> MAAPEAEVLSSAAVPDLEWYEKSEETHASQIELLETSSTQEPLNASEAFCPRDCMVPVVFPGPVSQEGCCQFTCELLKHIMYQRQQLPLPYEQLKHFYRKPSPQAEEMLKKKPRATTEVSSRKCQQALAELESVLSHLEDFFARTLVPRVLILLGGNALSPKEFYELD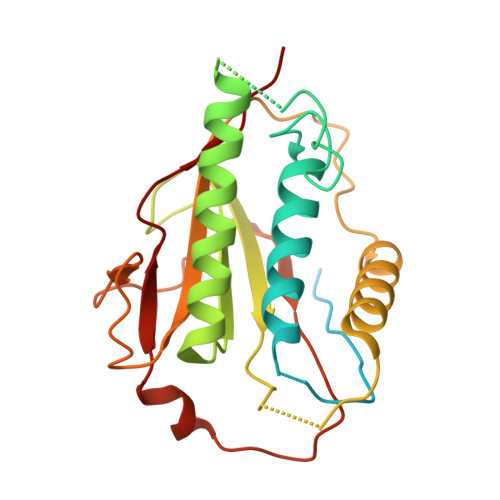LSLLAPYSVDQSLSTAACLRRLFRAIFMADAFSELQAPPLMGTVVMAQGHRNCGEDWFRPKLNYRVPSRGHKLTVTLSCGRPSIRTTAWEDYIWFQAPVTFKGFRE> RSVVGGLVALRGAHPYIAALYWGHSFCAGSLIAPCWVLTAAHCLQDRPAPEDLTVVLGQERRNHSCEPCQTLAV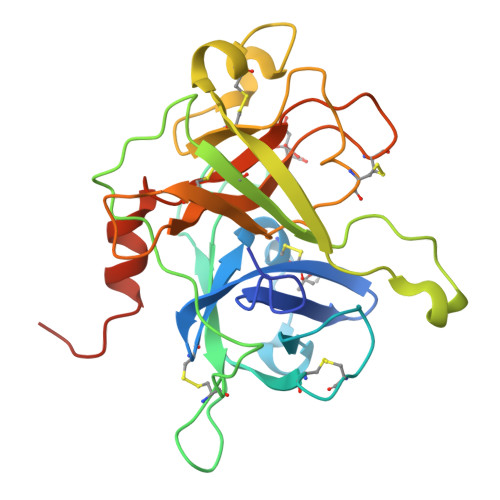RSYRLHEAFSPVSYQHDLALLRLQEDADGSCALLSPYVQPVSLPSGAARPSETTLCQVAGWGHQFEGAEEYASFLQEAQVPFLSLERCSAPDVHGSSILPGMLCAGFLEGGTDACQGDSGGPLVCEDQAAERRLTLQGIISWGSGCGDRNKPGVYTDVAYYLAWIREHTVSHHTGTRHHHHHH>MAMHPRKDWYELTRATNWTPSYVTEEQLFPERMSGHMGIPLEKWESYDEPYKTSYPEYVSIQREKDAGAYSVKAALERAKIYENSDPGWISTLKSHYGAIAVGEYAAVTGEGRMARFSKAPGNRNMATFGMMDELRHGQLQLFFPHEYCKKDRQFDWAWRAYHSNEWAAIAAKHFFDDIITGRDAISVAIMLTFSFETGFTNMQFLGLAADAAEAGDYTFANLISSIQTDESRHAQQGGPALQLLIENGKREEAQKKVDMAIWRAWRLFAVLTGPVMDYYTPLEDRSQSFKEFMYEWIIGQFERSLIDLGLDKPWYWDLFLKDIDELHHSYHMGVWYWRTTAWWNPAAGVTPEERDWLEEKYPGWNKRWGRCWDVITENVLNDRMDLVSPETLPSVCNMSQIPLVGVPGDDWNIEVFSLEHNGRLYHFGSEVDRWVFQQDPVQYQNHMNIVDRFLAGQIQPMTLEGALKYMGFQSIEEMGKDAHDFAWADKCK[2x];>[2x]MSFESKKPMRTWSHLAEMRKKPSEYDIVSRKLHYSTNNPDSPWELSPDSPMNLWYKQYRNASPLKHDNWDAFTDPDQLVYRTYNLMQDGQESYVQSLFDQFNEREHDQMVREGWEHTMARCYSPLRYLFHCLQMSSAYVQQMAPASTISNCCILQTADSLRWLTHTAYRTHELSLTYPDAGLGEHERE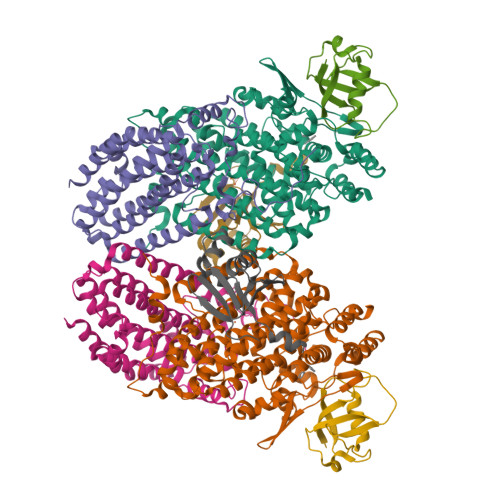LWEKEPGWQGLRELMEKQLTAFDWGEAFVSLNLVVKPMIVESIFKPLQQQAWENNDTLLPLLIDSQLKDAERHSRWSKALVKHALENPDNHAVIEGWIEKWRPLADRAAEAYLSMLSSD;>MSAFPVHAAFEKDFLVQLVVVDLNDSMDQVAEKVAYHCVNRRVAPREGVMRVRKHRSTELFPRDMTIAESGLNPTEVIDVVFEE[2x];>[2x]MSTLADQALHNNNVGPIIRAGDLVEPVIETAEIDNPGKEITVEDRRAYVRIAAEGELILTRKTLEEQLGRPFNMQELEINLASFAGQIQADEDQIRFYFDKTM>MFNNRIRTAALAGAIAISTAASGVAIPAFAQETGTYNNTGGFNDADGSTIQPAPAVDHSEAELRDATDATGNYLAAFQSGDIEAIVGAYIDAGVDGFDPSEEAIFKAFEAARDEATQQLAFSAETITKTRESVAYALKVDQEATEAYLAYRNALRGAATSINPLIDAANAANRTDGSEIEIYDNIFLASDVFTDGPLLLPAYRELVALQTEVNEDLEWLGEFAIDNDADNYVQRYHIPAVEALKAEIDARLEAIEPLRADSAEKNRLAQKSDVLVRQLFLERATAQRDTLRIVEAI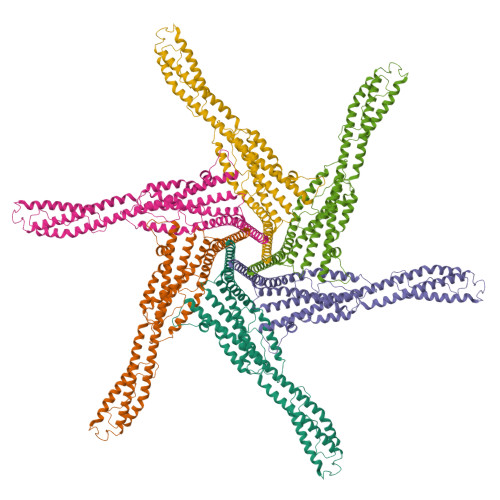FATATRYVELYESDEDVNVEGKTLREHYFALFPTLFGAASFNVGVLNTADDAVIDYYLVWDTDLETNDEDAAYAEEKREFALLTYAKIFINGQWQEKVKYVQNLDDGARAEAARIEAERLADEAYRAEQLRIAQEAADAQKAIADALAKEAENNNNSGGDNSSDDKGTGSSDIGSWGPFAAIAAIIAAIAAIFPFLSGIVKF[6x]> MAHHHHHHMKKILLVFGTRPEAIKMAPLVRALKARADVDAKVCVTAQHRQMLDQVLSLFDIEPDYDLDLMRQGQTLSDVTTGILHAIGAVFDDLRPDIVLVHGDTTTTLAVSLAAFYRYLPIGHVEAGLRSGDIWSPWPEELNRRVTDAVSSWHFAPTGQARDNLLSEGVPVGSVVMTGNTVIDALHDVKHMLERDDALSREVAARFPFLDPTARMVLITGHRRESFGEPFRNFCEALRTLAHRYRDAQFVYPLHLNPNVREPALALLGGEANIYLIEPQEYLAFVYLMSRSHFIITDSGGIQEEGPALGKPVLVTRDTTERPEAIRAGTARLVGTDPELIVREAS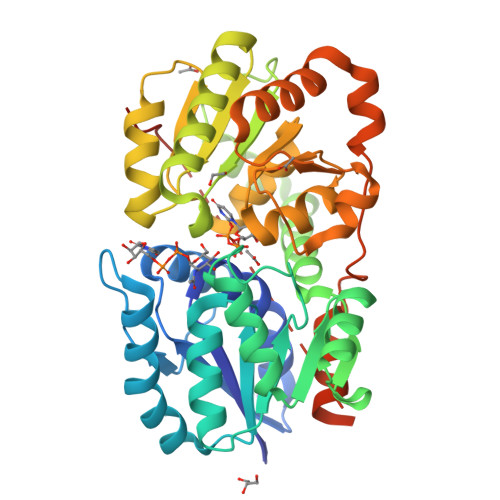RLFDSASAYDEMARASNPYGDGHASERIVHALMHTPASSANTTSFSMGAAELPLNALTLGLQALRSP> RPP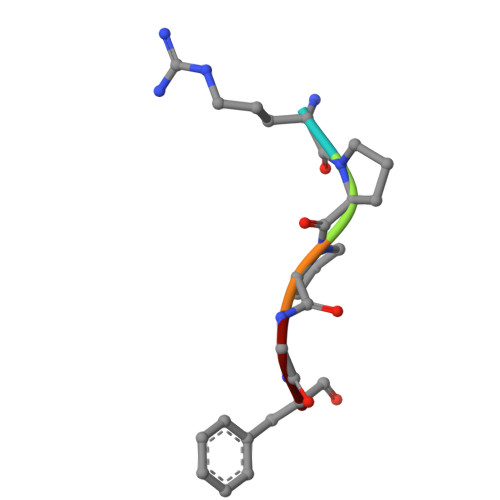GF>MKPVTLYDVAEYAGVSYQTVSRVVNQASHVSAKTREKVEAAMAELNYIPNRVAQQLAGKQSLLIGVATSSLALHAPSQIVAAIKSRADQLGASVVVSMVERSGVEACKTAVHNLLAQRVSGLIINYPLDDQDAIAVEAACTNVPALFLDVSDQTPINSIIFSHEDGTRLGVEHLVALGHQQIALLAGPLSSVSARLRLAGWHKYLTRNQIQPIAEREGDWSAMSGFQQTMQMLNEGIVPTAMLVANDQMALGAMRAITESGLRVGADISVVGYDDTEDSSCYIPPLTTIKQDFRLLGQTSVDRLLQLSQGQAVKGNQLLPVSLVKRKTTLAPNTQT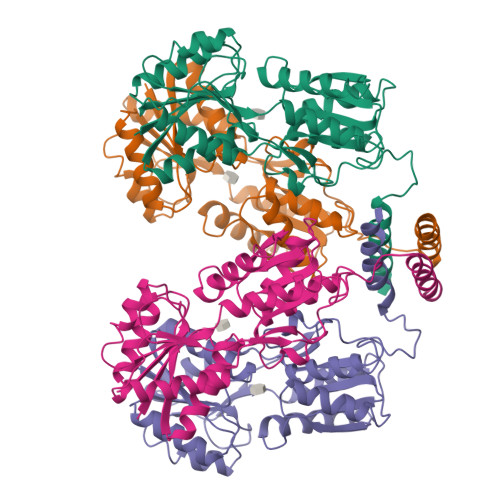ASPRALADSLMQLARQVSRLESGQ[4x]> GVDYKYKQKPKYQVRWKIIESYEGNSYTFIDPTQLPYNEKWEFPRNNLQFGKTLGAGAFGKVVEATAFGLGKEDAVLKVAVKMLKSTAHADEKEALMSELKIMSHLGQHENIVNLLGACTHGGPVLVITEYCCYGDLLNFLRRKSRVLETDPAFAIA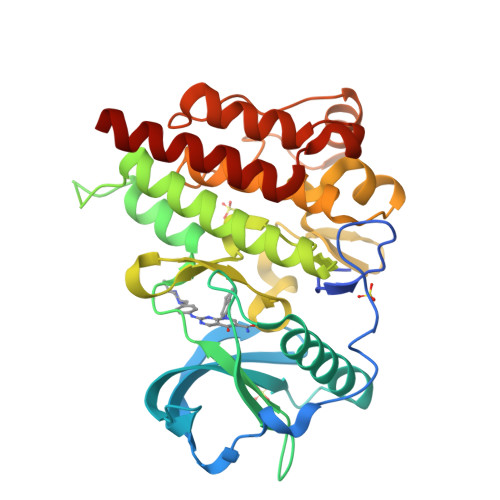NSTLSTRDLLHFSSQVAQGMAFLASKNCIHRDVAARNVLLTNGHVAKIGDFGLARDIMNDSNYIVKGNARLPVKWMAPESIFDCVYTVQSDVWSYGILLWEIFSLGLNPYPGILVNSKFYKLVKDGYQMAQPAFAPKNIYSIMQACWALEPTHRPTFQQICSFLQEQAQEDRRERD>[3x]MIHLYDAKSFAKLRAAQYAAFHTDAPGSWFDHTSGVLESVEDGTPVLAIGVESGDAIVFDKNAQRIVAYKEKSVKAEDGSVSVVQVENGFMKQGHRGWLVDLTGELVGCSPVVAEFGGHRYASGMVIVTGKGNSGKTPLVHALGEALGG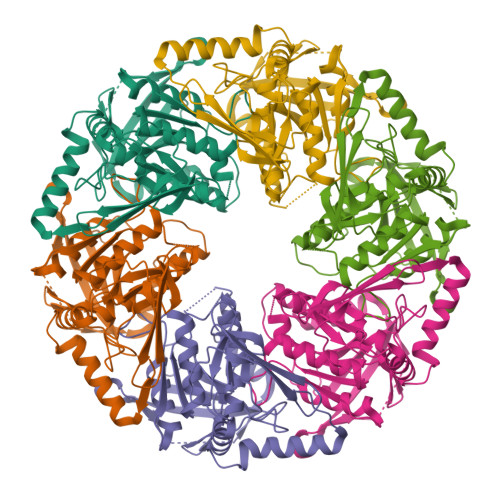KDKYATVRFGEPLSGYNTDFNVFVDDIARAMLQHRVIVIDSLKNVIGAAGGNTTSGGISRGAFDLLSDIGAMAASRGCVVIASLNPTSNDDKIVELVKEASRSNSTSLVISTDVDGEWQVLTRTGEGLQRLTHTLQTSYGEHAVLTIHTSKQSGGKQASGKAIQTVIKNDELESVLRRLTSN> GAMGYDYDYLFKIVLIGDSGVGKSNLLSRFTTDEFNIESKSTIGVEFATRTIEVENKKIKAQIWDTAGLERYRA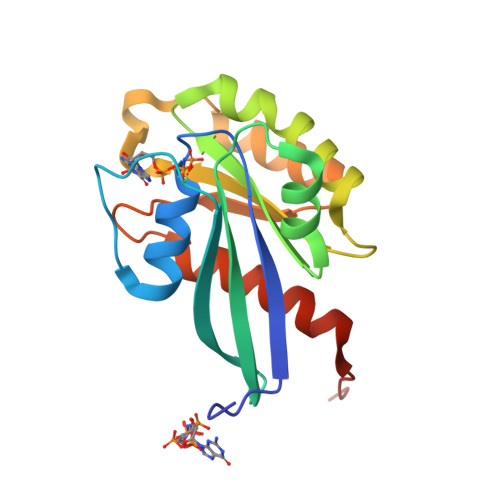ITSAYYRGAVGALIVYDISKSSSYENCNHWLTELRENADDNVAVGLIGNKSDLAHLRAVPTDEAKNFAMENQMLFTETSALNSDNVDKAFRELIVAIFQMVSKHQVDLSGS Caulobacter crescentus Tad (tight adherence) pili, part of the type IV pili family, are crucial for mechanosensing, surface adherence, bacteriophage (phage) adsorption, and cell-cycle regulation. Unlike other type IV pilins, Tad pilins lack the typical globular β sheet domain responsible for pilus assembly and phage binding. Furthermore, C. crescentus Tad pili are proposed as a phage receptor and indispensable for the infection of a single-stranded RNA (ssRNA) phage, ΦCb5 (14, 15). ΦCb5 carries a 3762-nt RNA genome encoding essential proteins, including a maturation protein (Mat), a coat protein (Coat), the β subunit of an RNA-dependent RNA replicase (Rep), and a lysis protein (Lys), with the gene lys embedded in the reading frame of the rep gene. In this study, we use single-particle cryo–electron microscopy (cryo-EM) to determine the molecular structure of the C. crescentus Tad pilus and comprehensively examine the molecular basis for the interaction between Tad pili and ΦCb5.

With our cryo-EM map of the ΦCb5 at a resolution of 2.7 Å, we reveal insights into the RNA packaging within the mature ΦCb5 virion and the arrangement of the Mat responsible for interacting with Tad pili. The ΦCb5 virion showcases a near-icosahedral spherical Coat shell of 89 Coat dimers with a diameter of around 290 Å, while a single Mat extends 30 Å beyond the shell. The gRNA adopts a defined conformation, presenting stem-loops to interact with the inner surface of the capsid. The Mat of ΦCb5 measures 135 Å long and 30 Å wide. It comprises a structural framework featuring a large β sheet including β strands β1 to β8, β10, and β11 and designated as the β region, as well as an α helix bundle, encompassing α helices α3 to α8 and designated as the α region. Positioned at a twofold axis of the capsid, the β region protrudes outward, while the α region penetrates deep into the capsid to bind the gRNA. In addition, we find that the N terminus of the Mat is exposed externally on the capsid, affording flexibility for potential protein tagging and engineering at this site. The gRNA density is overall gray except for the last 111 nucleotides (colored differently, including the last stem-loop of the replicase RNA gene and the 3′ untranslated region, or 3′UTR), which forms a four-way junction domain and interacts with the Mat. Stem-loop U1, the final RNA helix within the gRNA genome, engages in extensive interactions with the inner surface of Mat β region with its tip sandwiched between Mat and Coat dimer 2.

>[178x]ALGDTLTITLGGSGGTAKVLRKINQDGYTSEYYLPETSSSFRAKVRHTKESVKPNQVQYERHNVEFTETVYASGSTPEFVRQAYVVIRHKVGDVSATVSDLGEALSFYLNEALYGKLIGWES;> MARIRNRSSIASSGMSTFYLFGTPIVNEEIIVRNTEWCSDVIGNPGDNPLDIHKQEWTIKPLSGQIIFGSGTYRSLQCPPEYCRGASLSHLSLPSQSGLGTTALARTNPSRPAFNLPAFIGELRDLPRMFKIAGDTMLRKGANAFLSYQFGWKPLISDISKALDFSATVRTRSDEWHRLYSNGGLKRRINLGVDIEQKKENDVVLHSSNGFVVASHTVITVRKTWATVRWRPDAGSLPPITKSSSEKHARALLGLGVGGLIEGAWQLMPWSWMVDWFGNVGTFLQASNNTIGASPGLVNIMTTTTTNHQFSVKRDLSDGWIKGGDCSATVTSKARSQSSGPTITASIPNLSGRQLSILGALGIQRVPRHLLR> MRVTVSIIKADVGGFPGHAHVHPKMLEYAAAKLKEAQKRGVIIDYFVYNVGDDISLLMTHTKGEDNKDIHGLAWETFKEVTDQIAKRFKLYGAGQDLLKDAFSGNIRGMGPQVAEMEFEERPSEPIIAFAADKTEPGAFNLPLYKMFADPFTTAGLVIDPSMHEGFIFEVLDVVEHKVYLLKTPEDAYSLLGLIGTTGRYIIRKVFRRADGAPAAANSVERLSLIAGRYVGKDDPVLLVRAQSGLPAVGEVLEAFAHPHLVHGWMRGSHAGPLMPARFISVDPERRIAIGPKMTRFDGPPKVGALGFQLHEGYLEGGVDLFDDPAFDYVRQTAAQ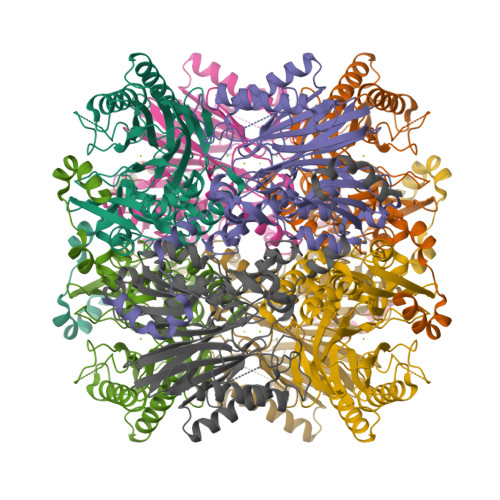IADYIRRMGPFQPHRLPPEEMEYTALPKILAKVKPYPADQYEKDRKKYIEAVVKGAKVEESQHDLEHHHHHH In response, one family of large bacteriophages uses a nucleus-like compartment to protect its replicating genomes by excluding host defence factors. Here we find that the bacteriophage nuclear shell assembles primarily from one protein, which we name chimallin (ChmA). Combining cryo-electron tomography of nuclear shells in bacteriophage-infected cells and cryo-electron microscopy of a minimal chimallin compartment in vitro, we show that chimallin self-assembles as a flexible sheet into closed micrometre-scale compartments. We find that the shell is primarily composed of a single protein, chimallin, which self-assembles through its extended N and C termini into a closed compartment.

Cryo-EM analysis of the 1.75 MDa assemblies revealed cubic particles approximately 22 nm in diameter, paralleling those formed by 201phi2-1 chimallin. We obtained a 4.2 Å-resolution structure of the overall Goslar chimallin assembly, and used a similar localized reconstruction procedure as for the 201phi2-1 chimallin to obtain a 2.6 Å-resolution structure of the Goslar chimallin tetramer, and a 2.3 Å-resolution structure of a single protomer. Overall, Goslar chimallin shows high structural homology to 201phi2-1 chimallin despite the low overall sequence identity, with a Cɑ r.m.s.d. of 1.8 Å within a protomer and 4.8 Å over an entire C4-symmetric tetramer. We performed cryoFIB–ET on E. coli cells infected with Goslar at mid-infection, followed by subtomogram analysis of phage nuclei. The resulting approximately 30 Å-resolution reconstruction showed high overall similarity to the structure of the 201phi2-1 nuclear shell, with a square grid of 11.5 × 11.5 nm units.

>SNAMGLDVRNNGNDNVEIRAAETRTAQRADEALETAADFAGQPKVTHTMRTINRTLSRRISRNTGSEQVLNLRRLMEKYLEDTRFKDDFIFVAVDPNQYSVPYPTLVVMSGAKVGDHNHFFGYVLPLVAGLAPLPRREEQGPHGNILVPRTWVDNLNGTFINEVMAAMYAAIGGKSNGTARIAGLAVVTNEITAESAHLATTLLSAADNAIQTAIEIRLGDKLGLPQFNLGMMASDQPISSVQYNTSGMQDSDIVGNPVRSDITVTISNRIRQAMSDYDSQQRLVATTGYIDLTYSPQNPTFNQGPVLVNGYPVPPTVQYQPRYVMTSAYPLELDAFTPNTFVLGLIGTIATLNSGMAWAQSLISNAARGIGPHNPGALAMVLDPEVTAPLDLSTQTNEQIYKFLQQVLYPSLLISIDVPEEGEYSWLLRMIPAAEKIYTGKVEGEVREISEGYKALYRAFDDVTLGCFSKKYQYGLPLVYATGNRIPLGHYNHQDGHRHDIRDMDDLYMMNITNPDTVEAWEDSFDRTDMTMSQRVVARHEIIDRVLSGSWEQTGWAMRYDFDPLALQALIEAAADAGFTIRPENIQHLAGTAVRGNMAARARGLGNISGNIYARSDRPNVGVNNMGGAFNLF[12x]> LSSNSSMNPKSLTDPKLLKNIPMWLKSLRLHKYSDALSGTPWIELIYLDDETL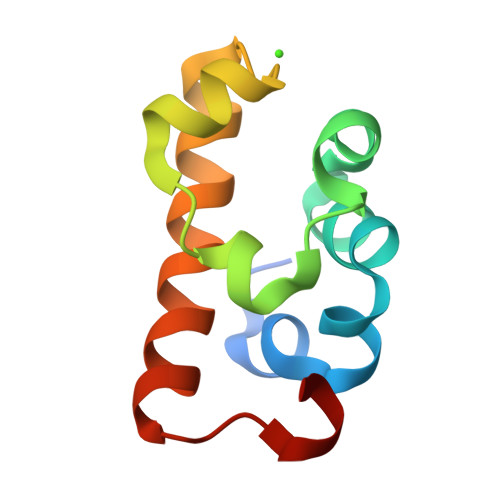EKKGVLALGARRKLLKAFGIVIDYKERDLIDRSAY> MALMQELYSTPASRLDSFVAQWLQPHREWKEEVLDAVRTVEEFLRQEHFQGKRGLDQDVRVLKVVKVGSFGNGTVLRSTREVELVAFLSCFHSFQEAAKHHKDVLRLIWKTMWQSQDLLDLGLEDLRMEQRVPDALVFTIQTRGTAEPITVTIVPAYRALGPSLPNSQPPPEVYVSLIKACGGPGNFCP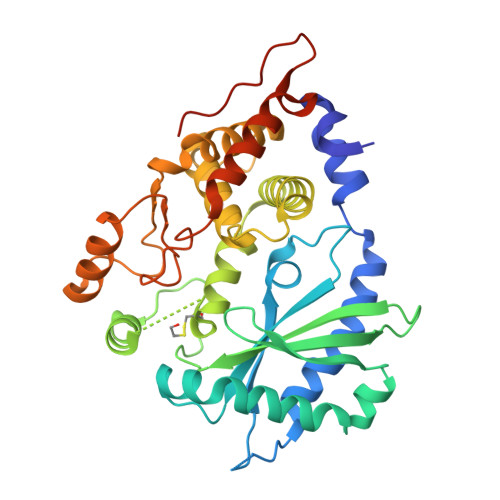SFSELQRNFVKHRPTKLKSLLRLVKHWYQQYVKARSPRANLPPLYALELLTIYAWEMGTEEDENFMLDEGFTTVMDLLLEYEVICIYWTKYYTLHNAIIEDCVRKQLKKERPIILDPADPTLNVAEGYRWDIVAQRASQCLKQDCCYDNRENPISSWNVKRGSSHHHHHH>MPSEQRGQHRSGYGLGLSTRTQVTGYQFLARRTAMALTRWRVRMEVEPGRRQVLAVVASVSAAGVICLGALLWSFISPSGQMGESPIIADRDSGALYVRVGDTLYPALNLASARLIAGRAENPHKVRSSQIAEQPHGPMVGIPGAPSDISPTSPASSSWLVCDAVTAAQGVGAPASVTVTVIDGTPDLSGRRHVLSGSDAVVLRYGNDTWVIRQGRRSRIDAANRAVLLPLGLTPEQVKQASPMSRALYDALPVGPELAVPKVPDAGKPANFPGAPAPVGAVLVTPQISGPQQYSVVLPDGVQTISPIVAQILQNAGTPAGSMPVVVAPATLARMPVVHGLDLSAYPDSPLNVVNMKENPATCWWWEKTAGEERARTQVVSGPTVPIATSDTNKVVSLVKADNTGREADRVYYGPNYANFVVVTGNDPAASTAESLWLLSKSGVRFGVDNSREARTALGLTSTPSPAPWVALRLLAPGPMLSRADALVRHDTLPTDTNPAELAVPK[6x];>[6x]MKQGFARPTPERAPVVKPENIVLPTPLSVPPPEGKPWWLVVVGVLVVGLLVGMVGMTVASGSRLFLGAGAIFPIFMIGGVAMMMFGGRFGGQQQMSRPKLDAMRAQFMLMLDMLRETAQESADSMDANYRWFHPAPTTLAAAVGSSRMWERQPDGKDLNFGVVRVGVGMTRPEVTWGEPQNMPTDIELEPVTGKALQEFGRYQSVVYNLPKMVSLLVEPWYSLVGEREQVLGLTRAIICQLAFSHGPDHVQMIVVTSDPDRWDWVKWIPHFGDPRRRDAAGNARMVYTSVREFATEQAELFAGRGSFTPRHASSSAETPTPHHVIISDIEDPQWEYVISSEGVDGVTFFDLTGSPLWTGAPQRVLRFTDSAGVIETLPRDRDTWMVIDDNAWFFALADQMSEADAEQFAHQMAHWRLAEAYEEIGQRVVQLGARDILSYYGIDDAGEIDFNTLWSGSGRRDLLSRSRLRIPFGNRADNGELLFLDMKSLDEGGDGPHGVMSGTTGSGKSSLVRTVIASLMLAHPPEELQFVLADLKGGSAVKPFDGVPHVSRIITDLEDDQALMERFLEAMWGEIARRKEICFSAGVDGAKEYNELRARMKARGEDMPPLPMLVVVIDEFYEWFRIMPTAVDVLDSIGRQGRAYWVHLMMASQTIESRAEKLMENMGYRLVLKAQTAGAAQAAGVPNAVNLPSQAGLGYFRKSGDEIIRFQAEYLWRDYRRGSSYDGEEQAPLTHSVDYIRPQLFTTAFAPLEVSVSGPDGQSALPQVVDGEAVNGHRGGDDVDEEEEALRTPKVGTVIIDQLRQIDFEPYRLWHPPLDVPVPIDELVNRFLGRPWQQDYGTAKNLVFPIGIIDRPYKHDQPPWTVDTSGAGANVLILGAGGAGKTTALQTLICAAALTHTPEQVQFYCLAYSGTALTTVANLPHVGGVSGPTDPYGVRRTVAEVLGLVRDRKRSFLEYDVPSMEVFRRRKFGGEPGGVPDDGFGDVYLVIDNYRALAEENEVLIEQVNQIINQGPSFGVHVVATADRESELRPPVRSGFGSRVELRLAAVEDAKLVRSRFAKDVPPKPGRGMVAVNYVRLDSDPQAGLHTLVARPALGSTPDAVFESDSVAAAVRQVAAGEARPVRRLPARFGLDQLRQVAAADRRQGVGAGGIAWAISELDLQPVYLNFADNAHLMVTGRRECGRTTTLATIMSEIGRIYAPGASTAPPTSRPSAQVWLVDPRRQLLTVLGSDYVEKFAYNLDGVAAMMDDLAAALARREPPPGLSAEELLSRSWWSGPEIFLIIDDIQQLPPGFDSPLHKAAPWVTRAADVGLHVFVTRTFGGWSSAGSDPILRALHQANAPLLVMDADPDEGFIRGKMKGGPLPRGRGLLMAEDTGVFVQVAATDLRR;>[12x]MTAIVEAPQPGAEAIASPQAAVVAIMAADVQIAVVLDAHAPISVMIDPLLKVVNTRLRELGVAPLEAKGRGRWMLCLVDGTPLRPNLSLTEQEVYDGDRLWLKFLEDTEHRSEVIEHISTAVATNLSKRFAPIDPVVAVQVGATMVAVGVLLGSALLGWWRWQHESWLPAPFAAVIAVLVLTVATMILARSKTVPDRRVGDILLLSGLVPLAVAIAATAPGPVGAPHAVLGFGVFGVAAMLVMRFTGRRLGVYTALVTLCAAATAAGLARMVLLTSAVTLLTCVLLACVLMYHGAPALSRWLSGIRLPVFPSATSRWVFEARPDLPTTVVVSGGGQPTLEGPASVRDVLLRAERARSFLTGLLVGLGVLTVVCLAGLCDPHAGRRWLPLLLAAFTFGFLILRGRSYVDRWQAITLAATAVLIIAAVAVR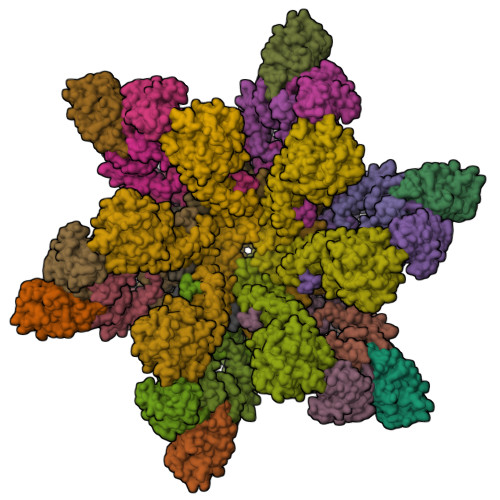YVLVSGSPAVLSAGVAVLVLLPAAGLTAAAVVPNTIYSPLFRKIVEWIEYLCLMPIFPLALWLMNVYEAIRYR;>MRAQRRFGLDLSWPRLTGVFLIDVAVLALVSHLPDAWQANHIAWWTGVGVAVLVTIVAVVTYRRTPLACALVARVLDRFVDPEMTLTEGCTPALDHQRRFGHDVVGIREYQGQLVAVVTVEGHEEAPSGRHRNRDAAPAWLPVEAVAARLRQFDVRLDAIDIVSVGTRRTSGRDDVSDVGVDDTGPVDARQPLDEHHTWLVLRMDPQRNVAAVAARDSVAATLAAATERLAHDLNGRRWTARPLTSSEIDDMDATVLAGLQPAHVRPRRRRLKYKQPEGYKEFVTSFWVSPRDITSETLERLWLPDTEATAVTVRLRPRHGGVEVSAWVRYHSSRRLRRSVWGGLNRLTGRQLDAVCASMPVPTRRPRLVVPARELHDGEELAVLVGQAPAPSPSPAAAR[6x]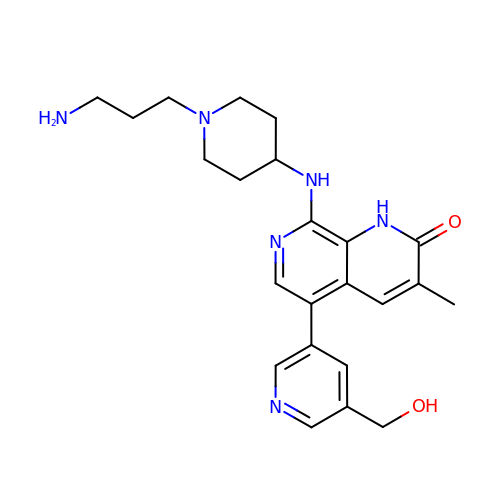8-[[1-(3-azanylpropyl)piperidin-4-yl]amino]-5-[5-(hydroxymethyl)pyridin-3-yl]-3-methyl-1~{H}-1,7-naphthyridin-2-one | C23 H30 N6 O2 | WQPQQRVHJTZSFA-UHFFFAOYSA-N>TKNITDAVAFAKSVKDVHTLVKSIDELA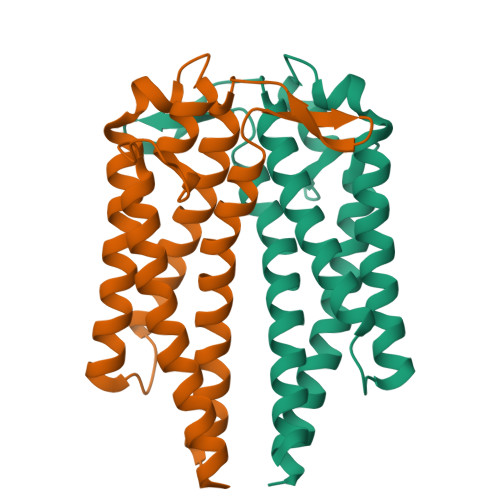KAIGKKIGANGLETDADKNAKLISGAYSVISAVDTKLASLEKKVGISDDLKGKITTVKNASTSFLTKAKSKTADLGKDDVKDADAKTAIDIADTGAKDKGAEELIKLNTAIDALLTSAEAAVTAAINALS[4x]Type I fungal FAS forms a barrel-shaped complex composed of two reaction chambers. Six β-chains form the walls of the barrel while a central wheel, made by the six α-chains, bisects the barrel into two chemically identical reaction chambers. Therefore, each chamber has three complete sets of catalytic domains including three acyl-carrier protein (ACP) domains. Substrates are shuttled between the static reaction centers by the mobile ACP domain flexibly tethered at its N and C termini.

In both our activity assays and cryoEM samples, the FAS enzymes were pre-incubated with cerulenin prior to addition of substrates acetyl- and malonyl-CoA and NADPH to ensure KS site was inhibited prior to the start of the reaction (i.e. KS-stalled state). In our high-resolution cryoEM maps, we can see appearance of additional densities immediately above the catalytic cysteine of the KS-domain in the KS-stalled state suggesting covalent linkage between cerulenin and the KS catalytic residue, which confirms our activity assay demonstrating inhibition of catalysis at the ketoacyl synthesis step. Stalling catalysis at the KS domain drastically alters the ACP densities inside the reaction chamber of both fungal FASs, as judged by improved ACP density near KS domain and weakened ACP density by the AT- and ER-domains in S. cerevisiae and C. albicans FASs, respectively. With the ability to observe ACP at the ER and redirect this mobile domain to the KS, we focused on conformational differences within the ER catalytic region of C. albicans FAS. This site within C. albicans enzyme represented the most pronounced alteration in ACP localization upon stalling catalysis at the KS-domain. In both species, the major improvement in cryoEM density of ACP at the stalled KS domain is observed at its canonical lobe. When ACP is shifted away from the ER domain in the KS-stalled state, the catalytic histidine is mainly in one conformation facing FMN. Weak density can be seen for the NADPH in proximity of FMN in the KS-stalled state, indicating partial/transient binding that does not clash with either of the histidine side chain conformations seen here. The observation that stalling catalysis at one site (i.e. KS) can affect ACP localization at other sites (i.e. AT and ER) in the presence of substrates within the context of the fully assembled reaction chamber strongly suggests that substrate loading state of the mobile domain may be a contributing factor in ACP-mediated substrate shuttling in type I fungal FAS.

> MKPEIEQELSHTLLTELLAYQFASPVRWIETQDVFLKQHNTERIIEIGPSPTLAGMANRTIKAKYESYDAALSLQRQVLCYSKDAKEIYYKPDPADLAPKETPKQEESTPSAPAAATPTPAAAAAPTPAPAPASAGPVESSSGAGSGAGAANSGGAVVDSAALDALTAENKKLAKQQLEVLARYLQVDLNKGSAKSFIKEKEASAVLQKELDLWEAEHGEFYAKGIQPTFSALKSRTYDSYWNWARQDVLSMYFDIIFGKLTSVDRETINQCIQIMNRANPTLIKFMQYHIDHCPEYKGETYKLAKRLGQQLIDNCKQVLTEDPVYKDVSRITGPKTKVSAKGNIEYEETQKDSVRKFEQYVYEMAQGGAMTKVSQPTIQEDLARVYKAISKQASKDSKLELQRVYEDLLKVVESSKEIETEQLTKDILQAATVPTTPTEEVDDPCTPSSDDEIASLPDKTSIIQPVSSTIPSQTIPFLHIQKKTKDGWEYNKKLSSLYLDGLESAAINGLTFKDKYVLVTGAGAGSIGAEILQGLISGGAKVIVTTSRFSKKVTEYYQNMYARYGAAGSTLIVVPFNQGSKQDVDALVQYIYDEPKKGGLGWDLDAIIPFAAIPENGNGLDNIDSKSEFAHRIMLTNLLRLLGAVKSKKTTDTRPAQCILPLSPNHGTFGFDGLYSESKISLETLFNRWYSEDWGSKLTVCGAVIGWTRGTGLMSANNIIAEGIEKLGVRTFSQKEMAFNILGLLTPEIVQLCQEEPVMADLNGGLQFIDNLKDFTSKLRTDLLETADIRRAVSIESAIEQKVVNGDNVDANYSKVMVEPRANMKFDFPTLKSYDEIKQIAPELEGMLDLENVVVVTGFAEVGPWGNSRTRWEMEAYGEFSLEGAIEMAWIMGFIKYHNGNLKGKPYSGWVDAKTQTPIDEKDIKSKYEEEILEHSGIRLIEPELFNGYDPKKKQMIQEVVVQHDLEPFECSKETAEQYKHEHGEKCEIFEIEESGEYTVRILKGATLYVPKALRFDRLVAGQIPTGWDARTYGIPEDTISQVDPITLYVLVATVEALLSAGITDPYEFYKYVHVSEVGNCSGSGMGGVSALRGMFKDRYADKPVQNDILQESFINTMSAWVNMLLLSSSGPIKTPVGACATAVESVDIGIETILSGKAKVVLVGGYDDFQEEGSYEFANMNATSNSIEEFKHGRTPKEMSRPTTTTRNGFMEAQGSGIQVIMTADLALKMGVPIHAVLAMTATATDKIGRSVPAPGKGILTTAREHHGNLKYPSPLLNIEYRKRQLNKRLEQIKSWEETELSYLQEEAELAKEEFGDEFSMHEFLKERTEEVYRESKRQVSDAKKQWGNSFYKSDPRIAPLRGALAAFNLTIDDIGVASFHGTSTVANDKNESATINNMMKHLGRSEGNPVFGVFQKYLTGHPKGAAGAWMLNGAIQILESGLVPGNRNADNVDKLLEQYEYVLYPSRSIQTDGIKAVSVTSFGFGQKGAQAVVVHPDYLFAVLDRSTYEEYATKVSARNKKTYRYMHNAITRNTMFVAKDKAPYSDELEQPVYLDPLARVEENKKKLVFSDKTIQSSQSYVGEVAQKTAKALSTLNKSSKGVGVDVELLSAINIDNETFIERNFTGNEVEYCLNTAHPQASFTGTWSAKEAVFKALGVESKGAGASLIDIEITRDVNGAPKVILHGEAKKAAAKAGVKNVNISISHDDFQATAVALSEF;> MSTHRPFQLTHGSIEHTLLVPNDLFFNYSQLKDEFIKTLPEPTEGFAGDDEPSSPAELYGKFIGFISNAQFPQIVELSLKDFESRFLDNNNDNIHSFAVKLLDDETYPTTIAKVKENIVKNYYKAVKSINKVESNLLYHCKHDAKLVAIFGGQGNTDDYFEELRELYTLYQGLIEDLLVSIAEKLNQLHPSFDKIYTQGLNILSWLKHPETTPDQDYLLSVPVSCPVICVIQLCHYTITCKVLGLTPGEFRNSLKWSTGHSQGLVTAVTIAASDSWDSFLKNSLTAVSLLLFIGSRCLSTYPRTSLPPTMLQDSLDNGEGRPSPMLSVRDLSIKQVEKFIEQTNSHLPREKHIAISLINGARNLVLSGPPESLYGFNLNLRNQKAPMGLDQSRVPFSERKLKCSNRFLPIFAPFHSHLLADATELILDDVKEHGLSFEGLKIPVYDTFDGSDFQALKEPIIDRVVKLITELPVHWEEATNHKATHILDFGPGGVSGLGVLTHRNKEGTGARIILAGTLDSNPIDDEYGFKHEIFQTSADKAIKWAPDWLKELRPTLVKNSEGKIYVKTKFSQLLGRAPLMVAGMTPTTVNTDIVSASLNAGYHIELAGGGYFSPVMMTRAIDDIVSRIKPGYGLGINLIYVNPFMLQWGIPLIKDLREKGYPIQSLTIGAGVPSIEVATEYIEDLGLTHLGLKPGSVDAISQVIAIAKAHPTFPIVLQWTGGRGGGHHSFEDFHQPIIQMYSKIRRCSNIVLVAGSGFGSDEDTYPYLSGYWSEKFNYPPMPFDGVLFGSRVMTSKESHTSLAAKKLIVECKGVPDQQWEQTYKKPTGGIITVRSEMGEPIHKIATRGVMFWKELDDTIFNLPKNKLLDALNKKRDHIIKKLNNDFQKPWFGKNANGVCDLQEMTYKEVANRLVELMYVKKSHRWIDVSLRNMYGDFLRRVEERFTSSAGTVSLLQNFNQLNEPEQFTADFFEKFPQAGKQLISEEDCDYFLMLAARPGQKPVPFVPVLDERFEFFFKKDSLWQSEDLESVVDEDVQRTCILHGPVASQYTSKVDEPIGDILNSIHEGHIARLIKEEYAGDESKIPVVEYFGGKKPASVSATSVNIIDGNQVVYEIDSELPNKQEWLDLLAGTELNWLQAFISTDRIVQGSKHVSNPLHDILTPAKHSKVTIDKKTKKLTAFENIKGDLLPVVEIELVKPNTIQLSLIEHRTADTNPVALPFLYKYNPADGFAPILEIMEDRNERIKEFYWKLWFGSSVPYSNDINVEKAILGDEITISSQTISEFTHAIGNKCDAFVDRPGKATLAPMDFAIVIGWKAIIKAIFPKSVDGDLLKLVHLSNGYKMITGAAPLKKGDVVSTKAEIKAVLNQPSGKLVEVVGTIYREGKPVMEVTSQFLYRGEYNDYCNTFQKVTETPVQVAFKSAKDLAVLRSKEWFHLEKDVQFDVLTFRCESTYKFKSANVYSSIKTTGQVLLELPTKEVIQVGSVDYEAGTSYGNPVTDYLSRNGKTIEESVIFENAIPLSSGEELTSKAPGTNEPYAIVSGDYNPIHVSRVFAAYAKLPGTITHGMYSSASIRALVEEWAANNVAARVRAFKCDFVGMVLPNDTLQTTMEHVGMINGRKIIKVETRNVETELPVLIGEAEIEQPTTTYVFTGQGSQEQGMGMELYNSSEVAREVWDKADRHFVNNYGFSILDIVQNNPNELTIHFGGAKGRAIRDNYIGMMFETIGEDGALKSEKIFKDIDETTTSYTFVSPTGLLSATQFTQPALTLMEKAAYEDIKSKGLIPSDIMFAGHSLGEYSALSSLANVMPIESLVDVVFYRGMTMQVAVPRDELGRSNYGMVAVNPSRVSATFDDSALRFVVDEVANKTKWLLEIVNYNVENQQYVAAGDLRALDTLTNVLNVLKINKIDIVKLQEQMSIEKVKEHLYEIVDEVAAKSLAKPQPIDLERGFAVIPLKGISVPFHSSYLMSGVKPFQRFLCKKIPKSSVKPQDLIGKYIPNLTAKPFELTKEYFQSVYDLTKSEKIKSILDNWEQYE>[2x]MTLPPDAPSRHRLVHALERTADLLDILGGEDFKSRAYRSAARSLEELNEETPELLAREFTGIPKVGKGIAAELSDFARSGTFAPLEAAAGQLPPGLLDLLG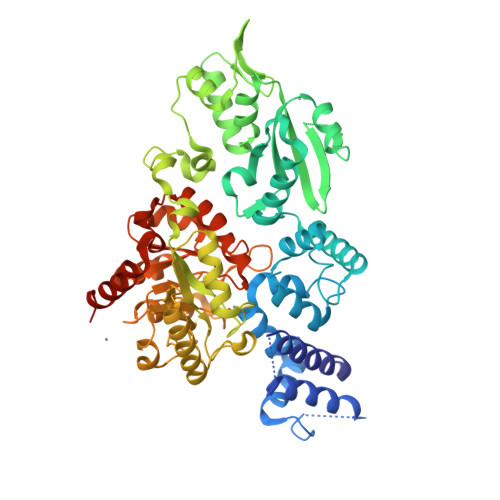VRGLGPKKIRSLWLAGIDSLERLREAAESGELAGLKGFGAKSAATILENVVFLFEARQRQSLRAGLAVAEELAGALTDLSPAPAGDVRRGLETVRAAELTVTGTPDDVLARLPELTVQGDGVLSGDYEGVPVEIACAPAEARGALDLLRSGEHFAGQVQAAAQARGFTLTAGGLSRGDEVLPTPTEAVVFHALDLPFRPAEYREPEHDDLWQTLPDPAELVTVGDLRGMIHTHSTWSDGGASIREMAEATLTLGHEFLGTADHSRAAYYANGLTIERLREQLKEIRELQRAGLPIVAGSEVDILDDGSLDFPDDVLGELDYVVVSVHSNFTLDAARQTERLIRAVSHPLVTVLGHATGRLLLRRPGYALDLDAVLGACEANGTVVEINANAARLDLDWREALRWRERLKFAINTDAHVPGGLRDARYGVMQARKAGLTPAHVVNSLGRAEFLDFVARQRAARGAPGPADRAHHHHHH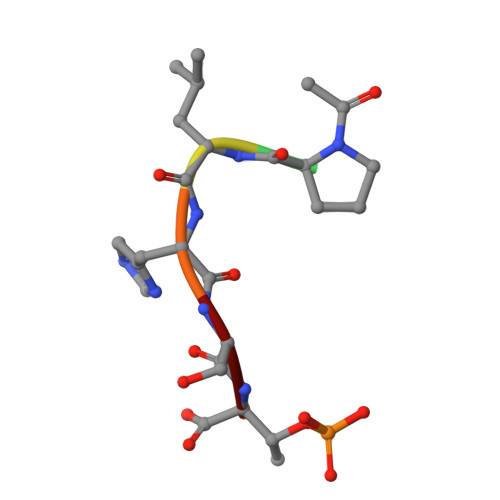> XPLHST methyl (R)-(6Z,9Z,12Z)-octadeca-6,9,12-trien-1-ylphosphonofluoridate | C19 H34 F O2 P | 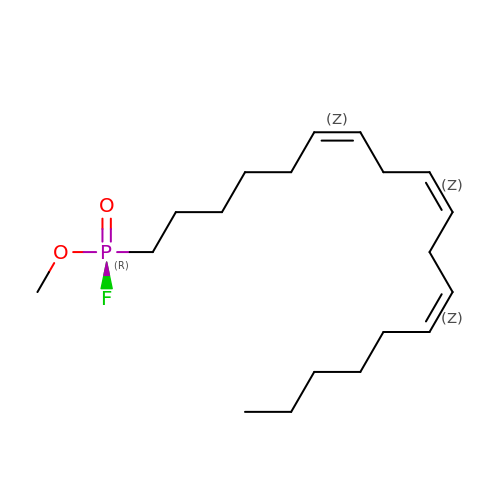PYIHGLSRUVHCML-YMLCEXCJSA-N>[3x]MDPYKEFGATVELLSFLPSDFFPSVRDLLDTASALYREALESPEHCSPHHTALRQAILCWGELMTLATWVGGNLEDGSGTSGSSGSGSGGSGSGGGGELSLLTEVETPIRNEWGSRSNDSSDDLSLLTEVETPIRNEWGSRSNDSSDDLSLLTEVETPIRNEWGSRS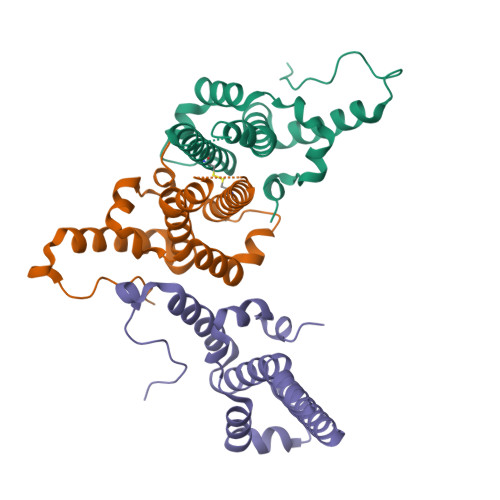NDSSDDLSLLTEVETPIRNEWGSRSNDSSDDIGTSGSSGSGSGGSGSGGGGGPSRDLVVSYVNTNMGLKFRQLLWFHISCLTFGRETVIEYLVSFGVWIRTPPAYRPPNAPILSTLPETTVC>[2x]MRGSHHHHHHGSDSELISENMHMKLYMEGTVNGHHFKCTSEGEGKPYEGTQTAKIKVVEGGPLPFAFDILATSFMYGSKTFINHTQGIPDFFKQSFPEGF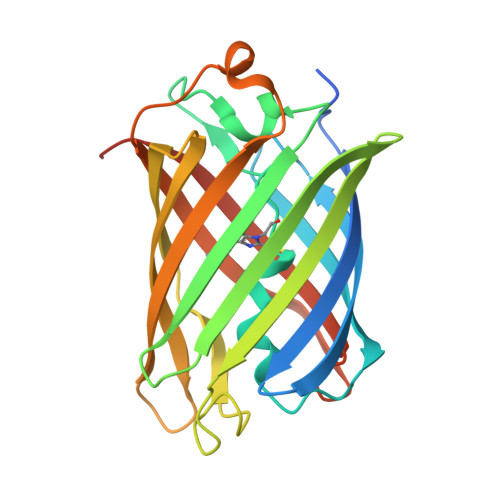TWERITTYEDGGVLTATQDTSLQNGCLIYNVKINGVNFPSNGPVMQKKTLGWEASTEMLYPADSGLRGHSQMALKLVGGGYLHCSLKTTYRSKKPAKNLKMPGFYFVDRKLERIKEADKETYVEQHEMAVARYCDLPSKLGHS> EQPEPIKVYGQVSLNDSHNQMVVHWAGEKSNVIVALARDSLALARPKSSDVYVSYDYGKSFKKISDKLNFGLGNRSEAVIAQFYHSPADNKRYIFADAYAQYLWITFDFCNTLQGFSIPFRAADLLLHSKASNLLLGFDRSHPNKQLWKSDDFGQTWIMIQEHVKSFSWGIDPYDKPNTIYIERHEPSGYSTVFRSTDFFQSRENQEVILE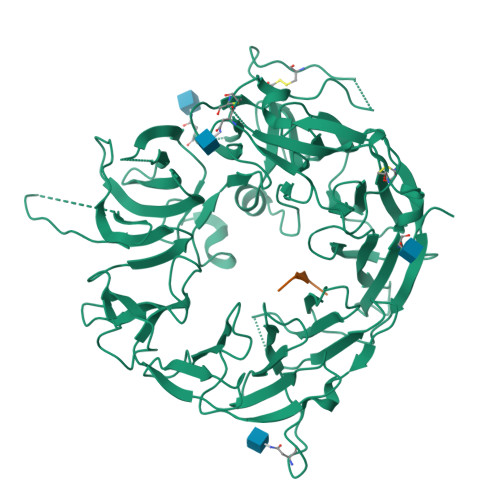EVRDFQLRDKYMFATKVVHLLGSEQQSSVQLWVSFGRKPMRAAQFVTRHPINEYYIADASEDQVFVCVSHSNNRTNLYISEAEGLKFSLSLENVLYYSPGGAGSDTLVRYFANEPFADFHRVEGLQGVYIATLINGSMNEENMRSVITFDKGGTWEFLQAPAFTGYGEKINCELSQGCSLHLAQRLSQLLNLQLRRMPILSKESAPGLIIATGSVGKNLASKTNVYISSSAGARWREALPGPHYYTWGDHGGIITAIAQGMETNELKYSTNEGETWKTFIFSEKPVFVYGLLTEPGEKSTVFTIFGSNKENVHSWLILQVNATDALGVPCTENDYKLWSPSDERGNECLLGHKTVFKRRTPHATCFNGEDFDRPVVVSNCSCTREDYECDFGFKMSEDLSLEVCVPDPEFSGKSYSPPVPCPVGSTYRRTRGYRKISGDTCSGGDVEARLEGELVPCPSRLENLYFQ;> AAAAAAAAAA1-(4-chloranylindol-1-yl)-2-methoxy-ethanone 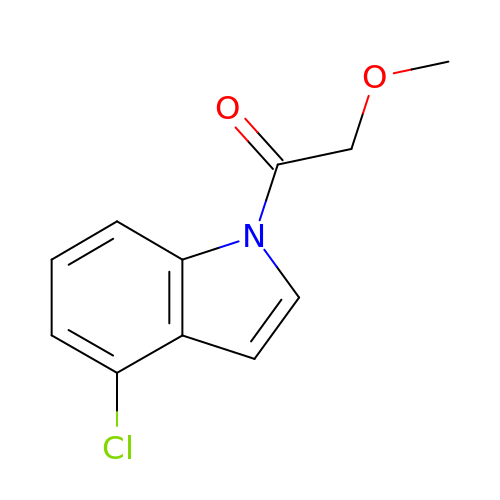| C11 H10 Cl N O2 | SLZGAMVJAWAHJX-UHFFFAOYSA-N> CNMWVIGKNKAQDAKAIMVNGPQFGWYAPAYTYGIGLHGAGYDVTGNTPFAYPGLVFGHNGTISWGSTAGFGDDVDIFAEKLSAEKPGYYQHNGEWVKMLSRKETIAVKDGQPETFTVWRTLHGNVIKTDTATQTAYAKARAWDGKEVASLLAWTHQMKAKNWPEWTQQAAKQALTINWYYADVNGNIGYVHTGAYPDRQPGHDPRLPVPGTGKWDWKGLLSFDLNPKVYNPQSGYIANWNNSPQKDYPASDLFAFLWGGADRVTEIDTTLDKQPRFTADQAWDVIRQTSRRDLNLRLFLPALKDATANLAENDPRRQLVDKLASWDGENLVNDDGKTYQQPGSAILNAWLTSMLKRTVVAAVPAPFGKWYSASGYETTQDGPTGSLNISVGAKILYEALQGDKSPIPQAVDLFGGKPQQEVILAALDDAWQTLSKRYGNDVTGWKTPAMALTFRANNFFGVPQAAAKEARHQAEYQNRGTENDMIVFSPTSGNRPVLAWDVVAPGQSGFIAPDGKADKHYDDQLIMYESFGRKSLWLTPQDVDEHKESQEVLQVQRLEH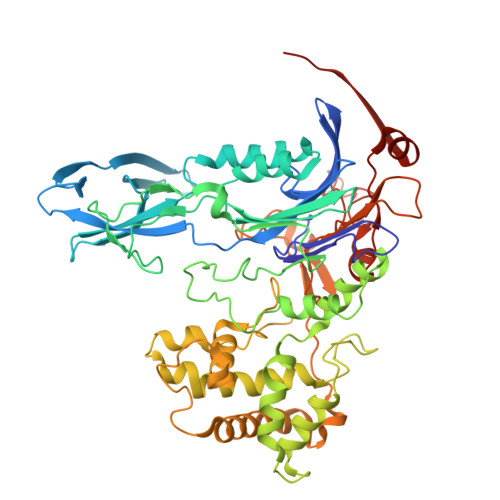HHHHH>MLAEKTRSIIKATVPVLEQQGTVITRTFYKNMLTEHTELLNIFNRTNQKVGAQPNALATTVLAAAKNIDDLSVLMDHVKQIGHKHRALQIKPEHYPIVGEYLLKAIKEVLGDAATPEIINAWGEAYQAIADIFITVEKKMYEEALWPGWKPFEITAKEYVASDIVEFTVKPKFGSGIELESLPITPGQYITVNTHPIRQENQYDALRHYSLCSASTKNGLRFAVKMEAARENFPAGLVSEYLHKDAKVGDEIK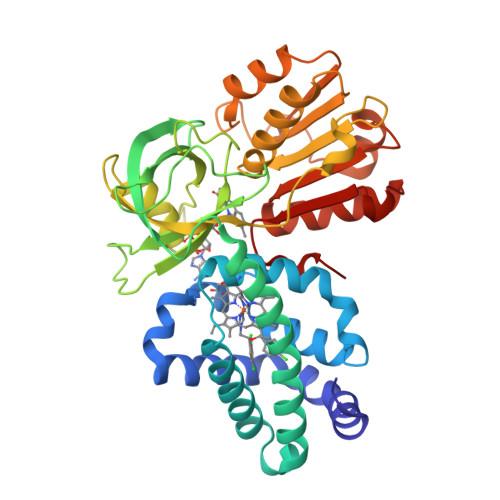LSAPAGDFAINKELIHQNEVPLVLLSSGVGVTPLLAMLEEQVKCNPNRPIYWIQSSYDEKTQAFKKHVDELLAECANVDKIIVHTDTEPLINAAFLKEKSPAHADVYTCGSLAFMQAMIGHLKELEHRDDMIHYEPFGPKMSTVQV[4x]> ATVIVVGLGIMGSATAWALARRGVRVVGLEQYAPFHALGSSHGKTRIIREAYFESPEYVPLVQRAYELWDELGERTGRRLLRVTGGVSIGRLDSPFIVGARESAQRHGLAHELLDAQEARKRFPVLALPDDFVALVEGRAGILFAEECWRAFCEDAVRHGAELRFGVRVHGFAPDGEGMTVETESGRLRADRVVVTAGPWS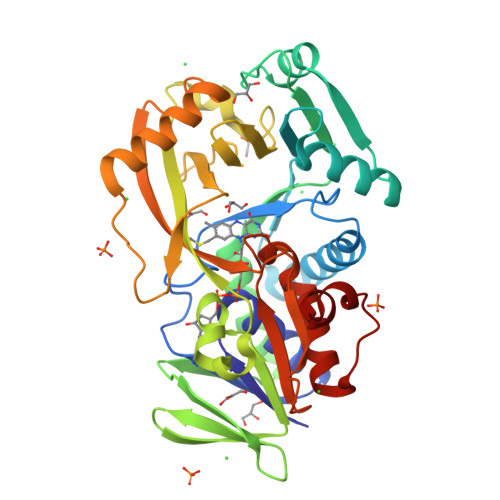TTLLADLGLPLEVRRVLVVHVQPDDPTRFRPEVLPIFIMDVPEGEYYGFPFLPDQGVKFGRHDDGEVCTPESVRRTVTDDEVRWMTGVLQRYLPGAAREVLMTVTCLYTMTPDRHFMIDRHPEWPQVVFAAGFSGHGFKFASVMGEALADLALEGASRLPIGFLSFRRLAK> MAVQFVNKQFNYKDPVNGVDIAYIKIPNVGQMQPVKAFKIHNKIWVIPERDTFTNPEEGDLNPPPEAKQVPVSYYDSTYLSTDNEKDNYLKGVTKLFERIYSTDLGRMLLTSIVRGIPFWGGSTIDTELKVIDTNCINVIQPDGSYRSEELNLVIIGPSADIIQFECKSFGHEVLNLTRNGYGSTQYIRFSPDFTFGFEESLEVDTNPLLGAGKFATDPAVTLAHELIHAGHRLYGIAI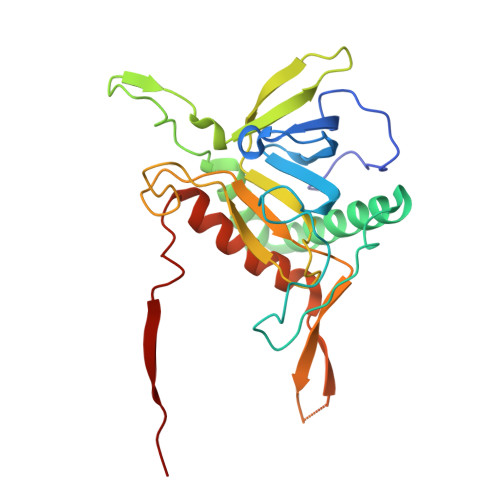NPNRVFKVNTNAY> XSIDMV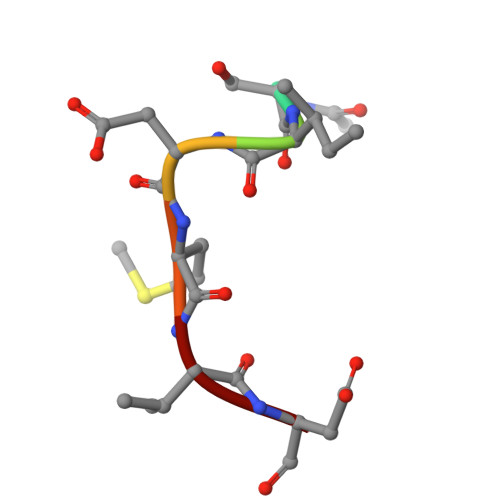D>[2x]QLFRALVSAQWVAEALKAPRSSQPLKLLDASWYLPKLGRDARREFEERHIPGAAFFDIDRSSDHTSPYDHMLPNATHFADYAGSLGVSAATHVVIYDGSDQGLYSAPRVWWMFRAFGHHSVSLLDGGFRHWLNQNLPISSGKSHSEPAE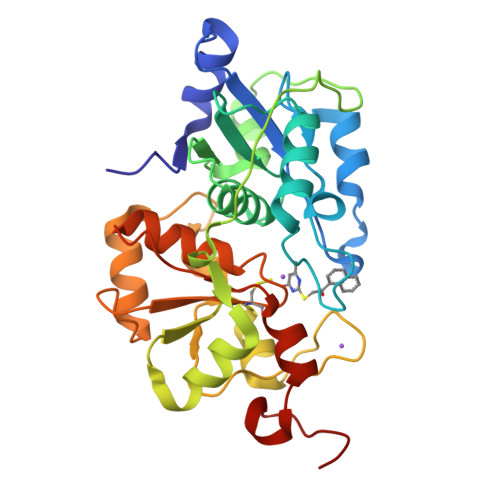FSAQLDPSFIKTHEDILENLDARRFQVVDARAAGRFQGTQPEPRDGIEPGHIPGSVNIPFTEFLTNEGLEKSPEEIKRLFKEKKVDLSKPLVATCGSGVTASHVVLGAFLSGKSDVPVYDGSWVEWYMRAQPEHIISEGRGKTQ>[2x]MAKTVETVLGPVPVEQLGKTL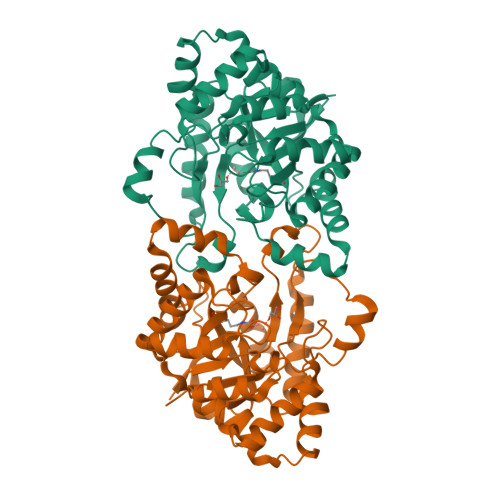IHEHFLFGYPGFQGDVTRGTFREDEALRVAVEAAEKMKRHGIQTVVDPTPNDCGRNPAFLRRVAEETGLNIICATGYYYEGEGAPPYFQFRRLLGTAEDDIYDMFMAELTEGIADTGIKAGVIKLASSKGRITEYEKMFFRAAARAQKETGAVIITHTQEGTMGPEQAAYLLEHGADPKKIVIGHMCGNTDPDYHRKTLAYGVYIAFDRFGIQGMVGAPTDEERVRTLLALLRDGYEKQIMLSHDTVNVWLGRPFTLPEPFAEMMKNWHVEHLFVNIIPALKNEGIRDEVLEQMFIGNPAALFSAHHHHHH> ANAFLEELRPGSLERECKEEQCSFEEAREIFKDAERTKLFWISYSDGDQCASSPCQNGGSCKDQLQSYICFCLPAFEGRNCETHKDDQLICVNENGGCEQYCSDHTGTKRSCRCHEGYSLLAD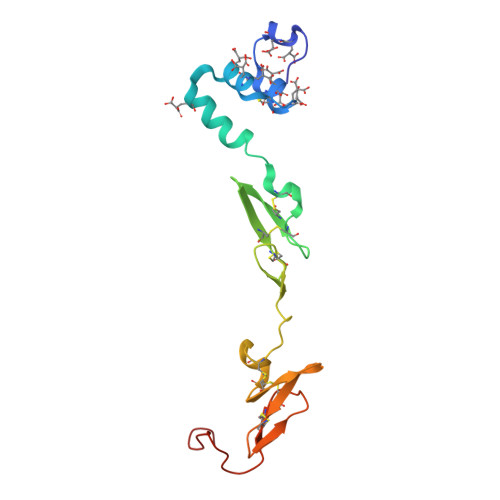GVSCTPTVEYPCGKIPILEK> MSQ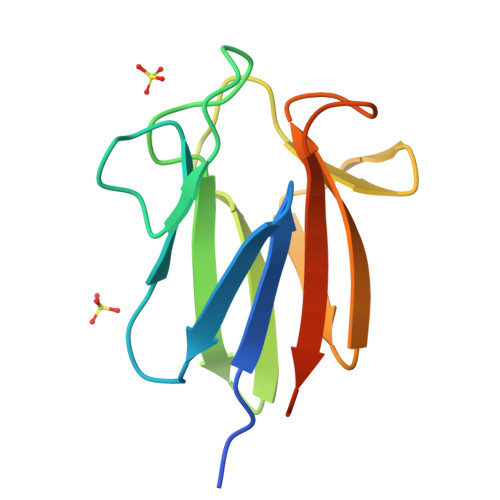PAAPPVLTVRYEGSERTFAAGHDVVVGRDLRADVRVAHPLISRAHLLLRFDQGRWVAIDNGSLNGLYLNNRRVPVVDIYDAQRVHIGNPDGPALDFEVGRHRGSAGRP> EQTSIAHLTSDDVNLPGSDFFRFYRSADKQEKEKARIYLLGVLDATEGKSWCQYSQLQTVTLQEFVFEFFNKLPAARLHERAAPLIEEALATRFPCKGGKA;> MKPLYRQLKSSHYSSDYSSPGYLAAEAVYAEIGYELDTLLKQNPGYANTCAVRM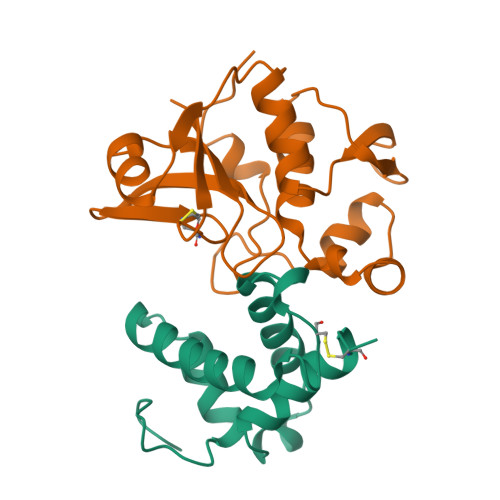SLALLKTGISFKGRLPIKKGAYKGKTIEPGAKLLADQLHRSSSFGKAKIFFNAPDAEKGIGNKKGVVFFNKITNYDGGHIDLIEPENSLLTCHSHCYFNCKEVWFWELS> MALNDNPIPKSVPLHPKSGKYFHNLHARDLSNIYQQCYKQIDETINQLVDSTSPSTIGIEEQV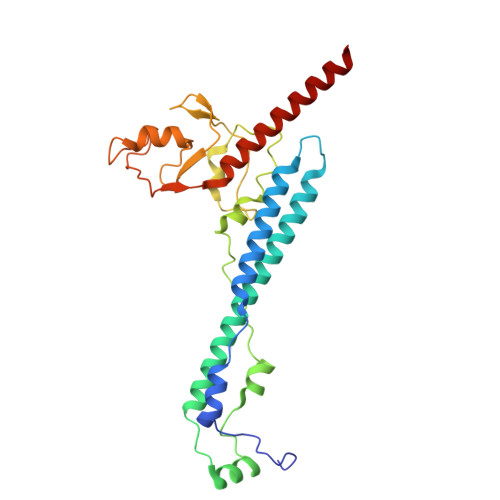ADITSTYKLLSTYESESNSFDEHIKDLKKNFKQSSDACPQIDLSTWDKYRTGELTAPKLSELYLNMPTPEPATMVNNTDTLKILKVLPYIWNDPTCVIPDLQNPADEDDLQIEGGKIELTCPITCKPYEAPLISRKCNHVFDRDGIQNYLQGYTTRDCPQAACSQVVSMRDFVRDPIMELRCKIAKMKESQEQDKRSSQAIDVL>RGHMPPLTSAQQALTGTINSSMQAVQAAQATLDDFETLPPLGQDAASKAWRKNKMDESKHEIHSQVDAITAGTASVVNLTAGDPAETDYTAVGCAVTTISSNLTEMSRGVKLLAALLEDEGGNGRPLLQAAKGLAGAVSELLRSAQPASAEPR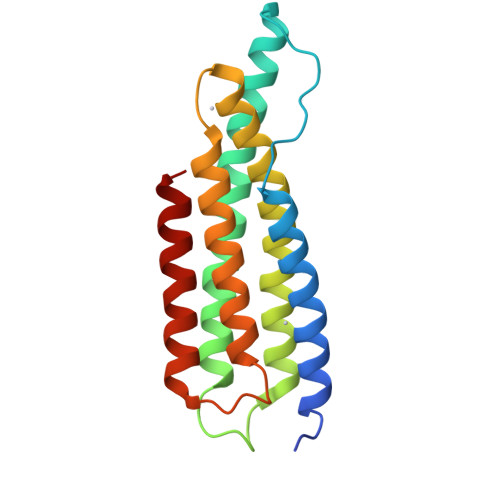QNLLQAAGNVGQASGELLQQI[3x]2-[4-(1,3-benzodioxol-5-ylmethyl)piperazin-1-yl]-N-[(1S,2S,5S)-2,5-dimethoxycyclohexyl]acetamide | C22 H33 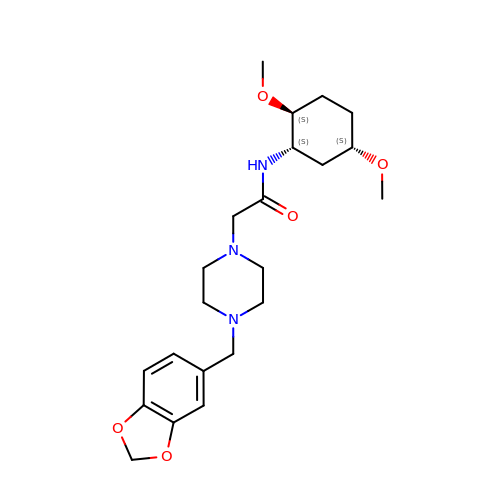N3 O5 | AOKPSAUXHJHABU-QYZOEREBSA-N> QDYGGKGMNVTQPPVVLASSRGVASFSCEYESSGKADEVRVTVLREAGSQVTEVCAGTYMVEDELTFLDDSTCIGTSRGNKVNLTIQGLRAMDT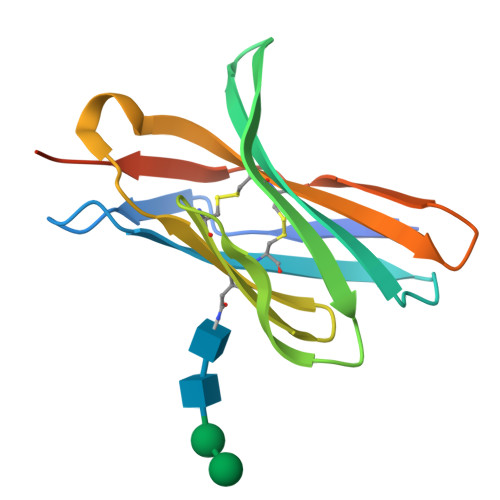GLYVCKVELMYPPPYYVGIGNGTQIYVIDPEPAENLYFQ> MKSVITTTISA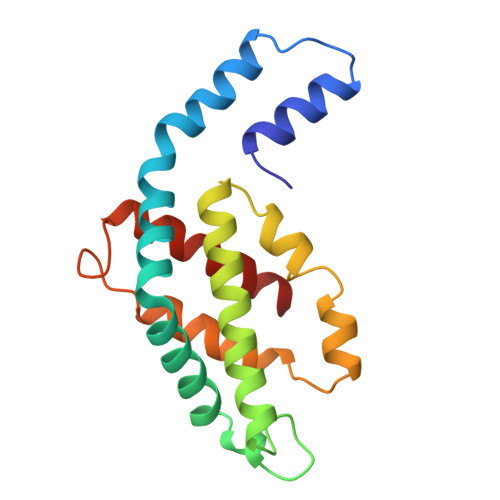ADAAGRFPSSSDLESIQGNIQRAAARLEAAQKLSGNHEAVVKEAGDACFAKYSYLKNAGEAGDSPEKINKCYRDIDHYMRLINYSLVVGGTGPVDEWGIAGSREVYRALNLPGSAYIAAFTFTRDRLCVPRDMSSQAGVEFTSALDYVINSLC> MQGGLFGTIKLMIMLFSYFAAYQLGKMQE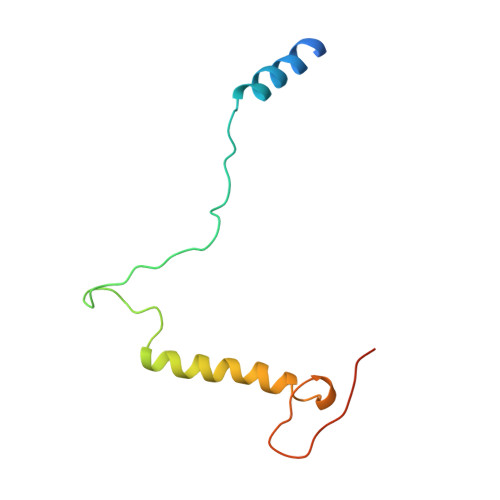RPQSQWPKAKAGQNKYMVGDWAAWKPIYMGVLGVAVLLTLLGPGGVGGGMGGMFGGGGGYGGYY>IDVEKLLELLIKAAAAEFTTYYYYTILRNHATGLEGEAIKEIIEDARLEDRNHFEALVPRIYELGGELPRDIREFADLASCRDAYLPEEPTIENILKVLLEAERCAVGVYTEICNYTFGKDPRTYDLALAILHEEIEHEAWFEELLTGKPSGHFRRGKPGESPYVSKFLK[12x]

The ferritin protein superfamily, nearly ubiquitous throughout the tree of life, has evolved to address iron storage, iron toxicity and free radical formation. ,, Ferritins oxidize Fe­(II) to Fe­(III) and store it within the ferritin nanoparticle as hydrated ferric oxyhydroxide. First identified in hyperthermophilic archaea, DPSL forms a 12-subunit (dodecameric) nanocage that preferentially utilizes H2O2 as a substrate. ,,, For these reasons, DPSL was first perceived as a DPS-Like mini-ferritin. However, structural studies revealed a surprise; DPSL lacks the DPS ferroxidase site and instead retains a bacterioferritin-like ferroxidase center in the middle of the 4-helix bundle. For these reasons, DPSL is proposed to lie at the evolutionary interface between the mini- and maxi-ferritins. ,− Importantly, DPSL further differentiates itself from both the (bacterio)­ferritins and DPS by the presence of two conserved cysteine residues that are juxtaposed between the ferroxidase center and the exterior surface of the particle. Together, the conserved cysteines and the bacterioferritin-like ferroxidase center serve as hallmarks of the archaeal DPSL proteins that are easily identified within the sequence as a “thioferritin” motif, and serve to differentiate DPSL as a distinct member of the ferritin superfamily.

Following incubation with 50 iron atoms per cage and stoichiometric amounts of H2O2 for 10 min, native mass spectrometry on intact protein cages indicated an average mass of 257 032 Da. Relative to the unloaded particles (256 118 Da), this was a mean increase of 913.6 Da, corresponding to approximately 10 Fe­(O)­OH units per cage. The overall structure of the iron nucleated particle is largely similar to the unmineralized structure, with a Cα RMSD of 0.37 Å. However, within the pore, we were able to model 11 iron atoms and 19 oxygen atoms in a 3-fold symmetric structure. Moving along the 3-fold axis from the interior of the particle outward, the six oxygen layers are stacked in an ABCACA manner, with the four innermost layers (ABCA···) resembling a cubic close-packed structure (ccp), while the 4 outer layers (..CACA) are instead hexagonal close-packed (hcp). Residues in the 3-fold channel that interact with the mineralized iron include Leu47, Glu50 and Glu54. However, in contrast to these prepositioned main chain carbonyl groups, the carboxylate side chains of Glu50 and Glu54 are rotated away from the nucleation site in the unmineralized structure, implying subsequent movement of these side chains into the nucleated conformation as the reaction proceeds. Overall, we see that DPSL utilizes a preformed, 3-fold symmetric crucible that is rich in precisely positioned carboxylate side chains and unsaturated main chain carbonyls.> MASIAVCPGSFDPVTYGHLDIIKRGAHIFEQVYVCVLNNSSKKPLFSVEERCELLREVTKDIPNITVET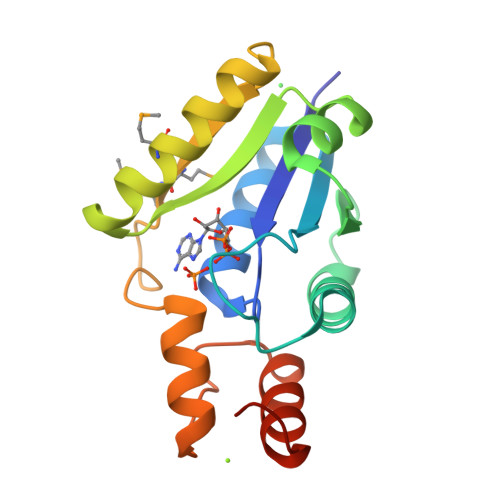SQGLLIDYARRKNAKAILRGLRAVSDFEYEMQGTSVNRVLDESIETFFMMANNQYSFLSSSIVKEVARYDGSVSEFVPPEVELALQQKFRQGGSHHHHHH N-(1-methyl-1H-pyrazol-3-yl)-2-(1H-pyrazol-1-yl)acetamide 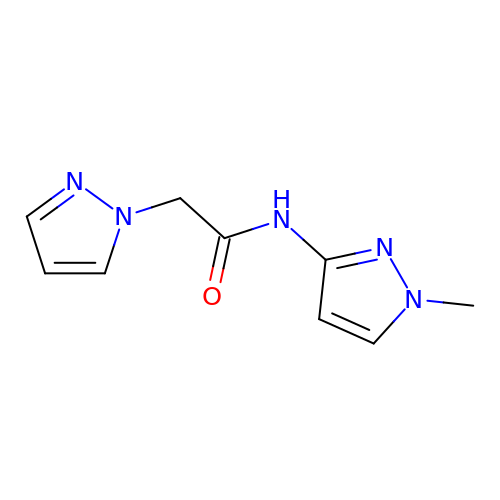| C9 H11 N5 O | DEBBFOBAIIGVSG-UHFFFAOYSA-N> YV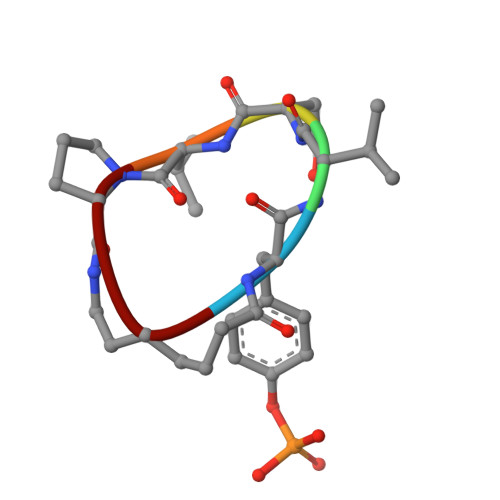NVPX> STGSATTTPIDSLDDAYITPVQIGTPAQTLNLDFDTGSSDLWVFSSETTASEVDGQTIYTPSKSTTAKLLSGATWSISYGD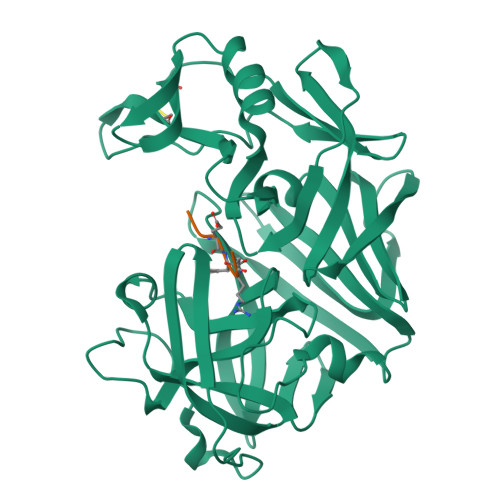GSSSSGDVYTDTVSVGGLTVTGQAVESAKKVSSSFTEDSTIDGLLGLAFSTLNTVSPTQQKTFFDNAKASLDSPVFTADLGYHAPGTYNFGFIDTTAYTGSITYTAVSTKQGFWEWTSTGYAVGSGTFKSTSIDGIADTGTTLLYLPATVVSAYWAQVSGAKSSSSVGGYVFPCSATLPSFTFGVGSARIVIPGDYIDFGPISTGSSSCFGGIQSSAGIGINIFGDVALKAAFVVFNGATTPTLGFASK;> PLEFRL> QSSTVGPNVVVAADGSGDYK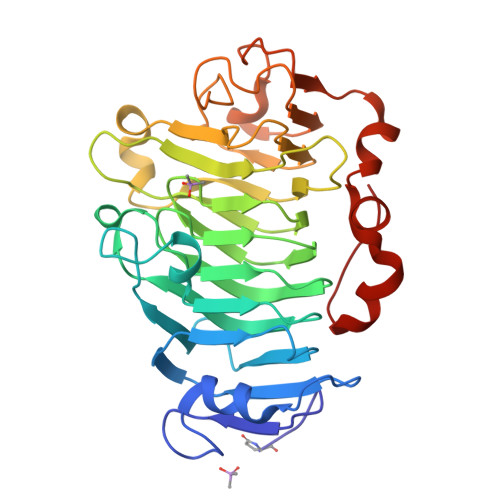TVSEAVAAAPEDSKTRYVIRIKAGVYRENVDVPKKKKNIMFLGDGRTSTIITASKNVQDGSTTFNSATVAAVGAGFLARDITFQNTAGAAKHQAVALRVGSDLSAFYRCDILAYQDSLYVHSNRQFFINCFIAGTVDFIFGNAAVVLQDCDIHARRPGSGQKNMVTAQGRTDPNQNTGIVIQKSRIGATSDLQPVQSSFPTYLGRPWKEYSRTVVMQSSITNVINPAGWFPWDGNFALDTLYYGEYQNTGAGAATSGRVTWKGFKVITSSTEAQGFTPGSFIAGGSWLKATTFPFSLGL8-[3,5-difluoro-4-(morpholin-4-ylmethyl)phenyl]-2-(1-piperidin-4-yl-1H-pyrazol-4-yl)quinoxaline | C27 H28 F2 N6 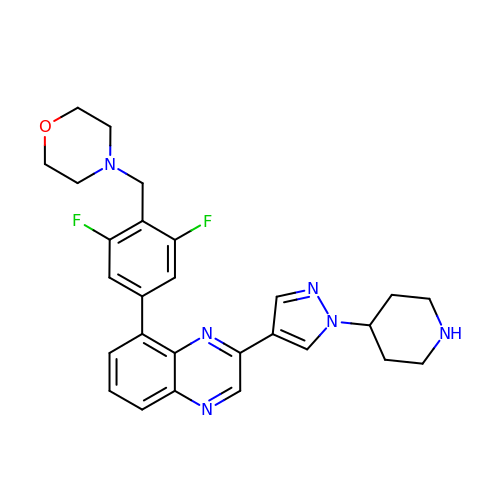O | IBPVXAOOVUAOKJ-UHFFFAOYSA-N> MKHHHHHHMTFPGDTAVLVLAAGPGTRMRSDTPKVLHTLAGRSMLSHVLHAIAKLAPQRLIVVLGHDHQRIAPLVGELADTLGRTIDVALQDRPLGTGHAVLCGLSALPDDYAGNVVVTSGDTPLLDADTLADLIATHRAVSAAVTVLTTTLDDPFGYGRILRTQDHEVMAIVEQTDATPSQREIREVNAGVYAFDIAALRSALSRLSSNNAQQELYLTDVIAILRSDGQTVHASHVDDSALVAGVNNRVQLAELASELNRRVVAAHQLAGVTVVDPATTWIDVDVTIGRDTVIHPGTQLLGRTQIGGRCVVGPDTTLTDVAVGDGASVVRTHGSSSSIGDGAAVGPFTYLRPGTALGADGKLGAFVEVKNSTIGTGTKVPHLTYVGDADIGEYSNIGASSVFVNYDGTSKRRTTVGSHVRTGSDTMFVAPVTIGDGAYTGAGTVVREDVPPGALAVSAGPQRNIENWVQRKRPGSPAAQASKRASEMACQQPTQPPDADQTP

The Rv1018c (glmU) gene product of Mycobacterium tuberculosis is an N-acetylglucosamine-l-phosphate uridyltransferase (GlmU). GlmU, a bifunctional enzyme, catalyzes the final two steps (reactions 1 and 2 below) in the de novo biosynthesis of UDP-GlcNAc from acetyl-CoA, glucosamine-1-phosphate and UTP, While the N-terminal domain of GlmU catalyzes uridyltransferase activity (reaction 2 above), acetyltransferase activity (reaction 1 above) at the C-terminal domain requires the formation of a bio­logical trimer. UDP-GlcNAc is an essential precursor for the biosynthesis of peptidoglycan and lipopolysaccharide, which are constituents of the bacterial cell wall. GlmU consists of two domains: an N-terminal uridyltransferase domain with an α/β-like fold and a C-terminal acetyltransferase domain that forms a left-handed parallel β-helix structure (LβH) with the shape of an equilateral triangular prism consisting of ten turns.

GlmU crystals in the ligand-free state were grown in VDX plates (Hampton Research) by the hanging-drop vapour-diffusion method at 277 K against 1 ml reservoir solution consisting of 25 mM MES pH 6.5, 1.8 M ammonium sulfate, 5% glycerol, 5 mM MgCl2. The crystals belonged to the cubic space group I432, with unit-cell parameters a = b = c = 285.7 Å, and contained one molecule per asymmetric unit. The GlmU crystals belonged to space group I432 (No. 211) and contained one molecule per asymmetric unit with a solvent content of ∼82%. With one molecule per asymmetric unit, the monomers from three neighbouring asymmetric units related by the crystal threefold formed a biological trimer. Although this is the first report of the structure of GlmU determined in a cubic crystal form, the trimeric arrangement here is similar to that observed for other GlmU structures determined in hexagonal (H3, H32, P6322) space groups. Although GlmU consists of 495 amino acids, a model could only be built for residues 1–472. The extended C-­terminus present in M. tuberculosis GlmU was not well defined in the electron-density map. The residues 149–150, 154–158, 164–177 and 200–206 that are part of the N-terminal active site are not well defined in the electron-density maps as the active site is devoid of bound ligands. The biological trimer found in the current structure of GlmU is similar to that in the GlmU homologues, except that the active-site residues 398–403 are disordered. Therefore, it appears that the tail-to-tail arrangement of trimers in the cubic form results in a sparse packing in the cubic crystal form of GlmU.>MANDSVSLTSNISNTSGVLLESQTKITDGALHFDGKKLNHNTFENPSKSQAYDYFFGRNISAHGDAVKPYKHFVFMTWYKGGKEERNVMLSRFNTKTGVVKTIQFPHRHTGFRGDPLVGESHNTIGLAVSPLNGTIHMVYDMHAYVDDDETGRFKGRFVDDFFRYSFSVAGAADVPDDEFTLEQFVKDTSELSQGADDYKHLTMTGNLQDKENFSALTYPKFYTSDDGELLHYMNWGGNNNGAYYFNKYDAKNQKWTRFTPFNHKDQKTHGNAYNWGLYGQMKYINGKLRVGFQQRSANNDDRFKYQNGVYYAYSDHPDGLG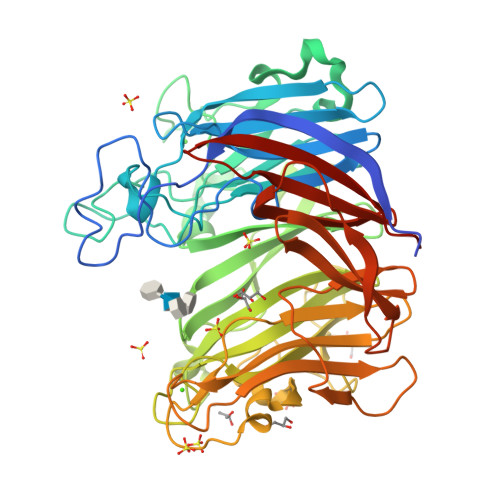NWKNVDGEDMTWPLVNSDEIKIFEPGDYIDHTAPNSVHIVTGFDWTVTENDDVHFITHVRSTDTKRSDYKEVSIHAFKPANAVDFTITTDFTGADSIYTSGDSIFIIGLKNGYPFVEKAKGGSNDFEVVYQQASGVKFDHGTIHIENGKAYYYLMEKGAGNALPLHLQVIDLGVTELEHHHHHH[2x]7N-METHYL-8-HYDROGUANOSINE-5'-MONOPHOSPHATE | C11 H18 N5 O8 P | 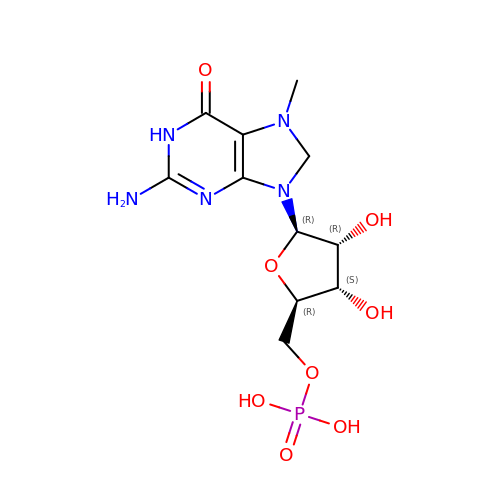ZMWJGXGSWZFZPJ-KQYNXXCUSA-N>[2x]MAHHHHHHSSGLEVLFQGPNTPVLEKNNVTLTGGGENVTKELKDKFTSGDFTVVIKYNQSSEKGLQALFGISNSKPGQQNSYVDVFLRDNGELGMEARDTSSNKNNLVSRPASVWGKYKQEAVTNTVAVVADSVKKTYSLYANGTKVVEKKVDNFLNIKDIKGIDYYMLGGVKRAGKTAFGFNGTLENIKFFNSA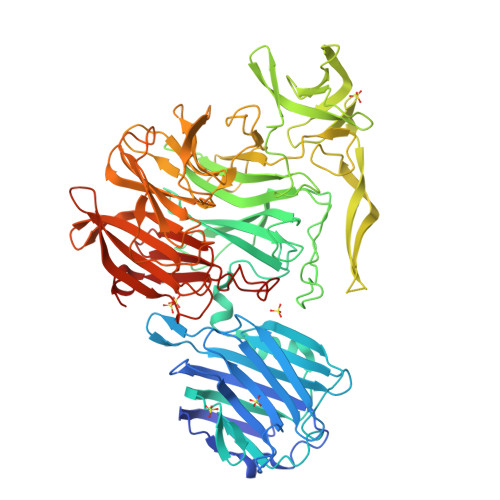LDEETVKKMTTNAVTGHLIYTANDTTGSNYFRIPVLYTFSNGRVFSSIDARYGGTHDFLNKINIATSYSDDNGKTWTKPKLTLAFDDFAPVPLEWPREVGGRDLQISGGATYIDSVIVEKKNKQVLMFADVMPAGVSFREATRKDSGYKQIDGNYYLKLRKQGDTDYNYTIRENGTVYDDRTNRPTEFSVDKNFGIKQNGNYLTVEQYSVSFENNKKTEYRNGTKVHMNIFYKDALFKVVPTNYIAYISSNDHGESWSAPTLLPPIMGLNRNAPYLGPGRGIIESSTGRILIPSYTGKESAFIYSDDNGASWKVKVVPLPSSWSAEAQFVELSPGVIQAYMRTNNGKIAYLTSKDAGTTWSAPEYLKFVSNPSYGTQLSIINYSQLIDGKKAVILSTPNSTNGRKHGQIWIGLINDDNTIDWRYHHDVDYSNYGYSYSTLTELPNHEIGLMFEKFDSWSRNELHMKNVVPYITFKIEDLKKN>[2x]AQCSVDIQGNDQMQFNTNAITVDKSCKQFTVNLSHPGNLPKNVMGHNWVLSTAADM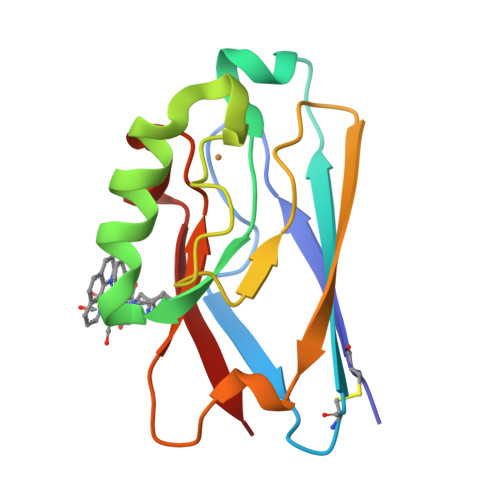QGVVTDGMASGLDKDYLKPDDSRVIAQTKLIGSGEKDSVTFDVSKLKEGEQYHFFCTFPGHSALMKGTLTLK>MGLNFFRKAAPEVRTEPVAERKASVTGRIVAMASGAGRPVWGPRDTVSLMRTGFAGNPVGFRSVKLIAEATAAVPLICQDAERRYEIHPVLDLLRRPNAGQGRAELFEALIGQILLSGNGYLEAVCPEPGVPRELHVLRSDRMAVVPGADGWPVGYDYTVGGRKHRFDMTGHPDPICHIKSFHPTDDHYGLSPMQAAAVALDVHNAASAWSKALLDNAARPSGAIIYKGADGQGVLAPEQYERLIFEMETHHQGARNAGRPMLLEGGLDWKPMGFSPSDMEFHETKAAAAREIALAFGVPPMLIGIPGDATYANYAEANRAFYRLTVLPLLTRVSAALAWWLSGYLGAQIELKPDLDQVPALAVERDQLWARIGAAGFLSNSEKRVLLGLPPTAEG[2x];>[11x]MDVFAKHAVSLESPAVRHYEITPSDSTDLARRPRALRVQTGGTLVLRDETGITVTYTVFAGEILPVRPVRVLATGTTATAVGWE;>MPEGADPVAEVKTALAGFLKEVKGFQDDVKTRLQQQEERVTMLQTKTYAGRHALAAAATEEAPHQKAFAAYLRTGDDDGLRGLSLEGKALNSAVAAEGGYLVDPQTSETIRGVLRSTASLRQIASVVNVEATSFDVLVDKTDMGSGWASETAALSETATPQIDRITIPLHELAAMPKASQRLLDDSAFDIETWLANRIADKFARAEAAAFISGDGVDKPTGFLTKTKVANGAWAWGSLGYVATGAAGDFAAVNASDAVVDLVYALGAEYRANASFVMNSKTAGAVRKMKDADGRFLWADSLAAGEPARLMGYPVLIAEDMPDIAANAYAIAFGDFGNGYTIAERPDLRVLRDPFSAKPHVLFYASKRVGGDVSDFAAIKLLKFAA[29x];>[2x]MMLNEVTAVPGTALPVAEFRDHLRLGTGFADLGAEDAALLSYLRAAIAAIEGRTAKALISRGFRLALTAWRWGDMQTLPIAPVATVTALRLVDAAGVETPVAAGWRLVPDMARPRIEALGAMLPMIPTGGRVEIDFTAGFGASWSALPVDLAQAVFLLAAQYYELRHDGAAEGGAMPFGVMALIERWRTVRVLGGRP;> MSRPRLNRLLVLEEAVRVADGAGGHRLDWQAKGEVWAEVTAGSGSERAGEFVTLASVPFTIVVRAAPVGAARRPRPEQRFREGARIFRILAVAERDREGHYLSCFAREEVVA;> MSYAVAGALQAAVYQQLRADAVLAALVGTAVYDAVPPGPLAGTYVSLGPEDVADASDKTGAGAVHDFVISVITDAAGFATAKAAAAAVSDALVGADLVLSRGRLVGLWFLRAKARRVEKADMRRIDLVFRARVEG;>MIALGLGLGLAANGGPALRRYAVNGVAPVAVLDFERHFLSHPLALTRATSATYADALRAVQTAPADTPRYDYSTGKRALLLEASATNLLPNSA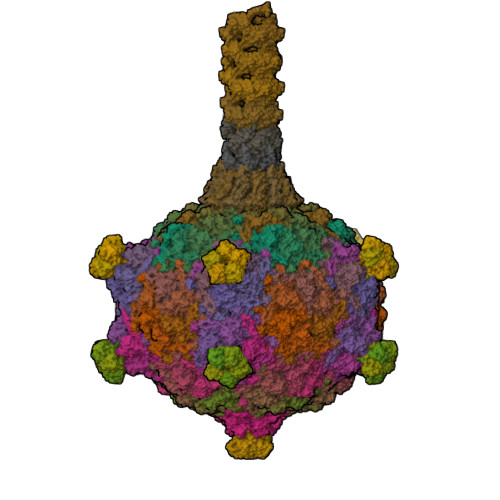QFEAASWGKTRASVLANAALAPNGTMTADKLVEDTSNNSHFVARTGTQIAAGTSVTASIFVKAAERRWFALVTADSANAFRTTYFDLQTGTLGVVSQGAAGHVAQIVAAGNGWYRCSVTQTQAASGNFNFYPSVASANGATSYPGDGASGLYLWGAQLEAGAAVSSVIPTEAAAVTRAADLASVAVAAGSYDLRRVDAAGTAVTKGVAHPGGALTIGAGSLYLLSLFPAGAL[2x];>MAAQNGKDLLIKLDLTGSGQFETIAGLRATRISFNAETVDVTSLESQGGWRELLGGAGVRSASISGAGVFKDADTDERARQIFFDGEVPEFQVIIPDFGIVQGPFMITSIDYAGSHNGEASYELAMASAGALSFTAI[4x]> GMPDIFQQEARGWLRCGAPPFAGAVAGLTTKHGGESKGPFASLNMGLHVGDDRTDVVNNRRRLAEWLAFPLERWVCCEQVHGADIQKVTKSDRGNGAQDFATAVPGVDGLYTDEAGVLLALCFADCVPIYFVAPSAGLVGLAHAGWRGTAGGIAGHMVWLWQTREHIAPSDIYVAIGPAIGPCCYTVDDRVVDSLRPTLPPESPLPWRETSPGQYALDLKEANRLQLLAAGVPNSHIYVSERCTSCEEALFFSHRRDRGTTGRMLAFIGRREEWT

Here, we report FAMIN as a prototype of a new family of multifunctional purine enzymes conserved from bacteria to man. FAMIN and its prokaryotic orthologs additionally have adenosine deaminase, purine nucleoside phosphorylase, and S-methyl-5′-thioadenosine phosphorylase activity, hence, combine activities of the namesake enzymes of central purine metabolism. Consistent with DUF152 containing all enzymatic activity, recombinantly expressed DUF152 bacterial proteins YlmD and YfiH metabolized adenosine to inosine and adenine, MTA to adenine, and inosine to hypoxanthine. Crystal structures of several bacterial DUF152 proteins have been determined and revealed a monomeric α/β/α fold (Kim et al., 2006).

The His47 side chain inserted into the purine-binding pocket in apo-YlmD (semi-transparent representation). The His47 side chain may act as a gatekeeper of the active site that rotates outward when the substrate binds. Atypical laccase activity has been ascribed to some bacterial DUF152 proteins based on a spectrophotometric method that monitors the oxidation of proxy substrates (Beloqui et al., 2006). In this method, YlmD, YfiH, and FAMIN254I, in contrast to a conventional laccase, elicited only minuscule signals. In a sensitive LC-MS method (Perna et al., 2018), laccase end-products were only detected with a conventional laccase but not with YlmD, YfiH, or FAMIN254I.>MAYFLDF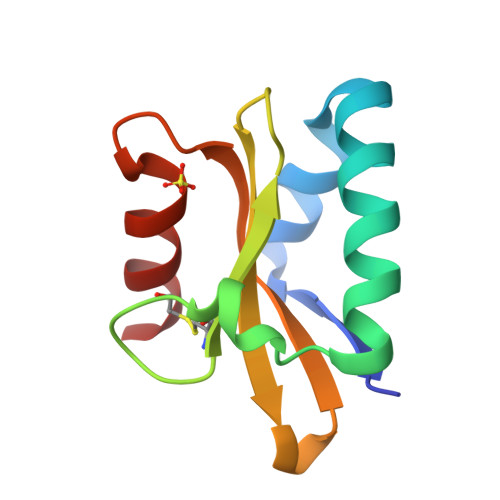DERALKEWRKLGSTVREQLKKKLVEVLESPRIEANKLRGMPDCYKIKLRSSGYRLVYQVIDEKVVVFVISVGKAERSEVYSEAVKRIL[3x]4-[4-[(dimethylamino)methyl]-3,5-dimethoxy-phenyl]-2-methyl-2,7-naphthyridin-1-one | C20 H23 N3 O3 | 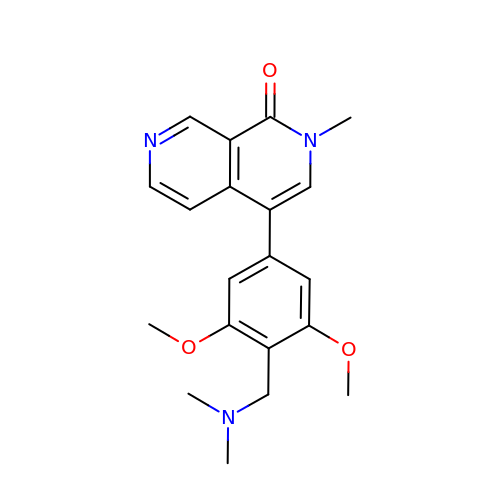RBUYFHLQNPJMQM-UHFFFAOYSA-N[(2R,3S,4R,5R)-5-(6-amino-9H-purin-9-yl)-3,4-dihydroxytetrahydrofuran-2-yl]methyl [(2R,3R,4R)-4-fluoro-3-hydroxytetrahydrofuran-2-yl]methyl dihydrogen diphosphate | C15 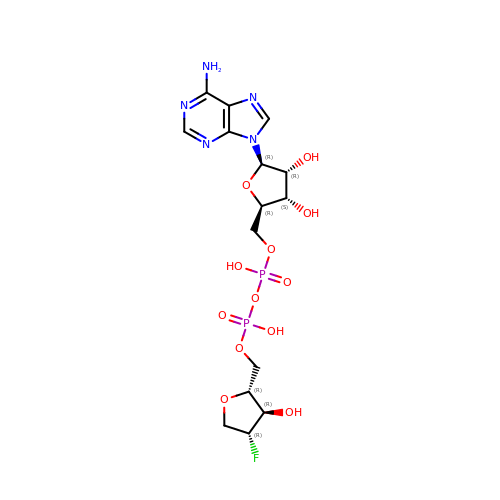H22 F N5 O12 P2 | GOCJJDZHXMDJEZ-WFCIOUKESA-N> VKWYYKTITFLPELCNNESLAAKCLRVLHGFNYQYETRNIGVSFPLWCDATVGKKISFVSKNKIELDLLLKQHYFVQMEQLQYFHISNTVLVPEDCTYVSFRRCQSIDKLTAAGLARKIRRLEKRALSRGEQFDPSSFAQKEHTAIAHYHSLGESSKQTNRNFRLNIRMLSEQPREGNSIFSSYGLSNSENSFQPVPLI;>[6x]GSMKLPTNLAYERSIDPSDVCFFVVWPDDRKTPLTYNSRTLLGQMEAASLAYDVSGQPIKSATAEALAQGNPHQVDFCHVPYGASHIECSFSVSFSSELRQPYKCNSSKVKQTLVQLVELYETKIGWTELATRYLMNICNGKWLWKNTRKAYCWNIVLTPWPWNGEKVGFEDIRTNYTSRQDFKNNKNWSAIVEMIKTAFSSTDGLAIFEVRATLHLPTNAMVRPSQVFTEKESGSKSKSKTQNSRVFQSTTIDGERSPILGAFKTGAAIATIDDWYPEATEPLRVGRFGVHREDVTCYRHPSTGKDFFSILQQAEHYIEVLSANKTPAQETINDMHFLMANLIKGGMFQHKGD;> MQTLKELIASNPDDLTTELKRAFRPLTPHIAIDGNELDALTILVNLTDKTDDQKDLLDRAKCKQKLRDEKWWASCINCVNYRQSHNPKFPDIRSEGVIRTQALGELPSFLLSSSKIPPYHWSYSHDSKYVNKSAFLTNEFCWDGEISCLGELLKDADHPLWNTLKKLGCSQKTCKAMAKQLADITLTTINVTLAPNYLTQISLPDSDTSYISLSPVASLSMQSHFHQRLQDENRHSAITRFSRTTNMGVTAMTCGGAFRMLKSGAKFSSPPHHRLNSKRSWLTSEHVQSLKQYQRLNKSLIPENSRIALRRKYKIELQNMVRSWFAMQDHTLDSNILIQHLNHDLSYLGATKRFAYDPAMTKLFTELLKRELSNSINNGEQHTNGSFLVLPNIRVCGATALSSP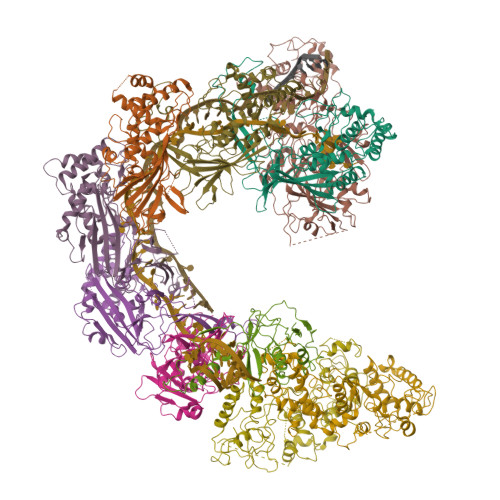VTVGIPSLTAFFGFVHAFERNINRTTSSFRVESFAICVHQLHVEKRGLTAEFVEKGDGTISAPATRDDWQCDVVFSLILNTNFAQHIDQDTLVTSLPKRLARGSAKIAIDDFKHINSFSTLETAIESLPIEAGRWLSLYAQSNNNLSDLLAAMTEDHQLMASCVGYHLLEEPKDKPNSLRGYKHAIAECIIGLINSITFSSETDPNTIFWSLKNYQNYLVVQPRSINDETTDKSSL;>[2x]MFLQRPKPYSDESLESFFIRVANKNGYGDVHRFLEATKRFLQDIDHNGYQTFPTDITRINPYSAKNSSSARTASFLKLAQLTFNEPPELLGLAINRTNMKYSPSTSAVVRGAEVFPRSLLRTHSIPCCPLCLRENGYASYLWHFQGYEYCHSHNVPLITTCSCGKEFDYRVSGLKGICCKCKEPITLTSRENGHEAACTVSNWLAGHESKPLPNLPKSYRWGLVHWWMGIKDSEFDHFSFVQFFSNWPRSFHSIIEDEVEFNLEHAVVSTSELRLKDLLGRLFFGSIRLPERNLQHNIILGELLCYLENRLWQDKGLIANLKMNALEATVMLNCSLDQIASMVEQRILKPNRKSKPNSPLDVTDYLFHFGDIFCLWLAEFQSDEFNRSFYVSRW Recently, a fluorophore named 5-((Z)-4-((2-hydroxyethyl)(methyl)amino)benzylidene)-3-methyl-2-((E)-styryl)-3,5-dihydro-4H-imidazol-4-one (NBSI), emitting in red spectrum, and its cognate aptamer named Clivia were identified, exhibiting a large Stokes shift. The overall structure uses a monomeric, non-G-quadruplex compact coaxial architecture, with NBSI sandwiched at the core junction. The overall structure of the complex adopts a coaxial long helix fold and is stabilized by continuous stacking interactions from the bottom stem P1 to the apical stem P2 with the ligand NBSI intercalated in the zipped junction region at the interface of stems P1 and P2. Our structural investigation of the Clivia aptamer bound to NBSI or NBSI derivatives revealed that the Clivia aptamer adopts a non-G-quadruplex scaffold supporting a specific ligand-binding pocket, suggesting a new fluorescence activation mechanism.

To enhance the imaging sensitivity of individual RNA molecules in the presence of a controlled concentration of fluorophore NBSI, we embarked on the design of constructs containing multiple NBSI-binding pockets arranged in tandem within a single sequence. Guided by the tertiary structure folding of monomeric Clivia, we used 3 bp from the north terminus of stem P1 and 2 bp from the south terminus of stem P2 as the linked stem. Therefore, the size of each NBSI-binding module in the multivalent Clivia fluorogenic aptamer was decreased from more than 36 nucleotides to 24 nucleotides. To detect whether the repeated NBSI-binding pockets were affected by the tandem-arrayed pattern, we set out to solve the complex structure of the multivalent Clivia fluorogenic aptamer bound to NBSI and succeeded with the Clivia_III construct containing three CM modules. The 5-bp linked stem between every two NBSI-binding modules was involved in A-minor interactions (A42 and A41) with the NBSI-binding pocket situated above it, as shown in the monomer structure. The residues lining each binding pocket were not affected by the tandem array of the NBSI-binding modules. Our in vitro experiment, coupled with structural research, revealed that these multivalent Clivia fluorogenic aptamers folded as homogeneous monomers in solution and each NBSI-binding module formed coaxially within the tertiary structure. Furthermore, we extended our exploration to the tertiary structure of the Clivia_III–NBSI complex, which contained three tandem arrays of Clivia fluorogenic modules.

>[2x]GGAAGAUUGUAAACAGCGAGAUUGUAAACAGCGAGAUUGUAAACAUGCCGAAAGGCAGACACUCGCGACACUCGCGACACUUUC>GGVEVLEVKTGVDAITEVECFLNPEMGDPDENLRGFSLKLSVQNDFSSDSPQRKMLPCYSTARIPLPNLNEDLTSGNLLMWEAVTVQTEVIGITSMLNLHAGSQKVHEHGGGKPIQGSNFHFFAVGGEPLEMQGVLMNYRSKYPDGTITPKNPTAQSQVMNTDHKAYLDKNNAYPVECWVPDPSRNENARYFGTFTGGENVPPVLHVTNTATTVLLDEQGVGPLCKADSLYVSAADICGLFTNSSGTQQWRGLARYFKIRLRKRSVKNPYP[5x]

BK polyomavirus (BKPyV) is a small, non-enveloped, double-stranded DNA virus with an icosahedral capsid formed by 72 capsomers, where a capsomer is an association of a pentamer of the VP1 protein linked internally to a single copy of either the VP2 or the VP3 proteins. BK polyomavirus (BKPyV) is an opportunistic pathogen that uses the b-series gangliosides GD1b and GT1b as entry receptors. Viruses sampled sequentially from these patients accumulated multiple mutations in the BC loop region of the VP1 protein, which is involved in the direct interaction of the virus with sialic acids. All variant VP1 pentamer structures were globally similar to the WT VP1 pentamer with a doughnut-shaped ring composed of a central pore surrounded by five VP1 monomers in 5-fold symmetry.

Interestingly, while the E73Q mutation on its own did not induce any structural changes, when combined with A72V, as seen in the VQQ variant, the second part of the BC loop was switched (RMSD of 2.8Å) in a similar manner to that seen in the E73A variant. However, in the case of the VQQ variant, the modified orientation of the BC loop was observed in all five VP1 monomers, not just in the two monomers seen in E73A. This suggests that mutations at position 73 on their own may not be enough to induce a clear structural change in the loop orientation, which only occurs if mutations in this position are combined with the A72V mutation at the neighboring amino acid. However, structural changes seen in the VQQ variant are not directly involved in the ganglioside interaction. Thus, the structure of the VQQ variant is consistent with its ability to bind gangliosides. VQQ VLPs were able to bind all gangliosides tested except GM1, confirming the glycan array data. Surprisingly, no infection was observed for VQQ in any supplementation condition, despite its ability to bind GD1b, GD1a, and other gangliosides on the surface of cells. Hence, ganglioside binding was not sufficient for infection with VQQ variant PSV. Variant VQQ showed broader ganglioside binding, but this was not sufficient for infectious entry in ganglioside-supplemented cells, clearly indicating the use of a co-receptor for the variant entry into cells. However, the VQQ variant retained some infectivity, suggesting that the interaction with this putative co-receptor was reduced, but not entirely abrogated, by the BC2 loop shift observed in the VQQ VP1 structure.The oxidative folding machinery in Gram-negative bacteria typically comprises a soluble periplasmic oxidase (disulfide bond protein A [DsbA]) and its partner membrane protein (disulfide bond protein B [DsbB]). Together with a quinone cofactor, DsbB generates de novo disulfide bonds which it donates to DsbA, which in turn oxidizes unfolded or partially folded substrate proteins. In the present study, we demonstrate that B. pseudomallei membrane protein disulfide bond protein B (BpsDsbB) forms a functional redox relay with the previously characterized virulence mediator B. pseudomallei disulfide bond protein A (BpsDsbA). In B. pseudomallei, deletion of dsbA has marked pleiotropic effects on virulence.

BpsDsbA in which the buried active-site cysteine (Cys 46) is mutated to alanine (BpsDsbAC46A) was incubated with a synthesized peptide of sequence Gly-Phe-Ser-Cys-Gly-Phe derived from residues 99 to 104 in the predicted periplasmic loop 2 of BpsDsbB. As a result of the active-site mutation, BpsDsbA cannot resolve the resulting intermolecular disulfide bond, creating a long-lived homogeneous complex suitable for crystallization. Accordingly, we determined the crystal structure of BpsDsbA in complex with a 6-mer peptide of BpsDsbB (GFSCGFBpspep) derived from periplasmic loop 2 of BpsDsbB (BpsDsbA-GFSCGFBpspep) in space group P1 using molecular replacement methods to 2.5 Å resolution. GFSCGFBpspep makes contacts with each of BpsDsbA's four catalytic surface loops. Its interaction with BpsDsbA is anchored by a central disulfide bond to the active site, and the flanking hydrophobic pocket contacts both Bpspep phenylalanine residues. Specifically, 102 Cys of the B. pseudomallei GFSCGF peptide (102 CysBpspep) is disulfide bonded to 43 Cys (2.04 Å) of BpsDsbA. 102 CysBpspep also makes two main-chain-mediated hydrogen bonds with the cis-Pro-1 residue 159 Val of L2. 100 PheBpspep is sandwiched in a pocket between BpsDsbA residues 176 Asn, 177 Ser, and 178 Leu (L3) and the side chain of the active-site residue BpsDsbA 45 His. Similarly, the phenyl ring of 104 PheBpspep inserts into a small hydrophobic pocket lined with BpsDsbA 73 Phe, 77 Phe, and 40 Trp. BpsDsbA-GFSCGFBpspep superimposes on apo WT BpsDsbA with an RMSD of 0.3 Å over 189 equivalent C-α atoms, and the catalytic surface loops are equivalently positioned.

>[4x]SNAAGFAQASPSAPVAGKDFEVMKSPQPVSAPAGKVEVIEFFWYGCPHAYEFEPTIEAWVKKQGDKIAFKRVPVAFRDDFVPHSKLFYALAALGVSEKVTPAVFNAIHKEKNYLLTPQAQADFLATQGVDKKKFLDAYNSFSVQGQVKQSAELLKNYNIDGVPTIVVQGKYKTGPAYTNSLEGTAQVLDFLVKQVQDKKL;>[4x]GFSCGF N-({(2S)-1-[(3R)-3-amino-4-(3-chlorophenyl)butanoyl]pyrrolidin-2-yl}methyl)-3-(methylsulfonyl)benzamide 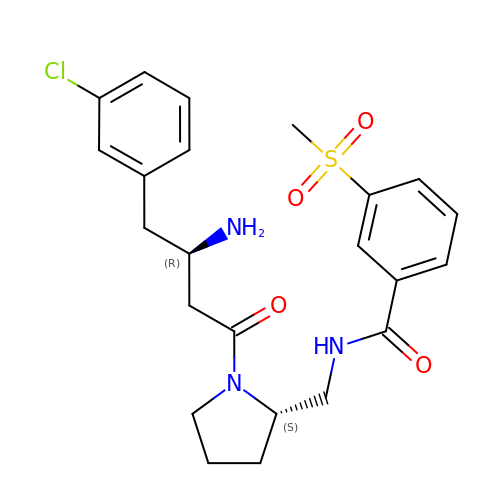| C23 H28 Cl N3 O4 S | QRGBOABBMKYMLG-UXHICEINSA-N> MSKLEAILSQEVEAEIQALLQEAEAKAEAVKREAEEKAKAL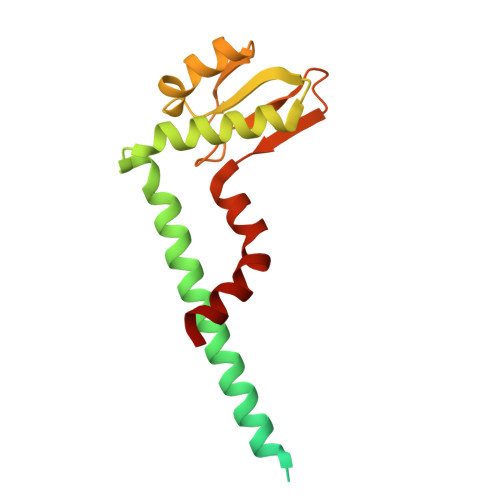LQARERALEAQYRAALRRAESAGELLVATARTQARGEVLEEVRRRVREALEALPQKPEWPEVVRKLALEALEALPGAKALVANPEDLPHLEALARERGVELQAEPALRLGVRAVGAEGKTQVENSLLARLDRAWDALSSKVAQALWG Arabidopsis thaliana (At) carboxylesterase 15 (CXE15) and carboxylesterase 20 (CXE20) have been shown to deplete strigolactones (SLs) that coordinate various growth and developmental processes and function as signaling molecules in the rhizosphere. Here, we elucidate the X-ray crystal structures of AtCXE15 (both apo and SL intermediate bound) and AtCXE20, revealing insights into the mechanisms of SL binding and catabolism. The N-terminal regions of CXE15 and CXE20 exhibit distinct secondary structures, with CXE15 characterized by an alpha helix and CXE20 by an alpha/beta fold. These structural differences play pivotal roles in regulating variable SL hydrolysis rates.

Similar to AtCXE15, the overall structure of AtCXE20 is divided into two domains: cap domain (residues 1–26) and the catalytic core domain (residues 53–327) both of which are also connected by a long linker loop (residues 27–52). The catalytic core of AtCXE20 adopts the common α/β hydrolase fold with eight-stranded β-sheet surrounded by 11 α-helices and one 310 helix. Unlike CXE15, CXE20 features a catalytic triad composed of Ser-His-Asp (instead of Ser-His-Glu), and both enzymes exhibit similar catalytic pockets, predominantly lined with hydrophobic residues. Strikingly, in contrast to AtCXE15, the cap domain of AtCXE20 comprises of NT α1 helix and anti-parallel β-sheet (β1 and β2), which we termed NT-α/β. Moreover, the loop connecting the NT-α/β to the core is longer in CXE20 compared to the loop connecting the NTH in AtCXE15 that is replaced by an extra β-strand. Additionally, CXE20 displays a short helix that connects the α9 and β9 regions, whereas this region is unstructured in CXE15. We found significant changes in the dimensions and biochemical compositions of the pocket where CXE15 exhibits a relatively compact cavity compared to CXE20 which has a deeper and wider cleft. The main difference between the pockets can be attributed to the presence of negatively charged and hydrophobic residues in CXE15, and positively charged and hydrophobic residues in CXE20. Notably, the presence of F31 and R307 in CXE20 may hinder the proper orientation of the ABC-ring of SLs and their dynamics resulted in larger pocket size (from 303 A2 to 620 A2), and can explain reduced enzymatic activity. CXE15 demonstrated much greater activity towards YLG hydrolysis than AtCXE20 with kcat values of 0.84 s−1 and 0.021 s−1, respectively.

>[2x]MSEPSPIADPYAYLNIVNNPDGSITRDLSNFPCTAATPDPSPLNPAVSKDLPVNQLKSTWLRLYLPSSAVNEGNVSSQKLPIVVYYHGGGFILCSVDMQLFHDFCSEVARDLNAIVVSPSYRLAPEHRLPAAYDDGVEALDWIKTSDDEWIKSHADFSNVFLMGTSAGGNLAYNVGLRSVDSVSDLSPLQIRGLILHHPFFGGEERSESEIRLMNDQVCPPIVTDVMWDLSLPVGVDRDHEYSNPTVGDGSEKLEKIGRLRWKVMMIGGEDDPMIDLQKDVAKLMKKKGVEVVEHYTGGHVHGAEIRDPSKRKTLFLSIKNFIFSVL>NLGAAVAILGGPGTVQGVVRFLQLTPERCLIEGTIDGLEPGLHGLHVHQYGDLTNNCNSCGNHFNPDGASHGGPQDSDRHRGDLGNVRADADGRAIFRMEDEQLKVWDVIGRSLIIDEGEDDLGRGGHPLSKITGNSGERLACGIIARSAGL[2x]

Superoxide dismutase-1 (SOD1) is one of the most abundant human proteins and is an important part of our antioxidant, redox signalling and respiratory control mechanisms. SOD1 folding, zinc and copper acquisition, and disulphide bond formation can be catalysed by the copper chaperone for SOD1 (CCS), which forms a transient heterodimeric complex with SOD1 to facilitate its maturation. Here, we discover the mechanisms that govern SOD1 maturation and stabilisation through interaction with the chaperone protein hCCS. Combinations of mutants yielded crystallographic structures of full-length hCCS in two different conformers complexed with hSOD1; an hCCS domain II truncation complexed with hSOD1; an hCCS domain II homodimer structure at higher resolution than previously available (1.55 Å); and the hSOD1 disulphide knock-out mutant used to promote complexation.

When homodimeric hSOD1 and hCCS domain II are physiologically zinc metalated, many of the terms that comprise binding free energy are equal due to their sequence and structural similarity. Indeed, orientation of monomers and the presence of four inter-subunit hydrogen bonds found in homodimeric hSOD1 are maintained by hCCS. The presence of a stabilising Coulombic interaction between opposing hCCS Arg104 and Asp136 residues (3.55 Å), which is not present in hSOD1, appears counterintuitive in this regard. However, the hCCS dimer interface is replete with positive charge and therefore not dominated by the hydrophobic effect seen in hSOD1 and many other protein complexes. Most importantly, however, the presence of hCCS Ala231 significantly weakens half of the homodimer interface hydrogen bonds conserved from SOD1. Specifically, Ala231 side-chain methyl pushes Arg232 and Gly135 apart through steric repulsion, lengthening the carbonyl-amine hydrogen bond between them to 3.08 Å from 2.75 Å, in the case of the homologous SOD1 residues Ile151 and Gly51. Without this rearrangement, hCCS Ala231 Cβ would be an energetically unfavourable 2.3 Å from the Gly135 carbonyl oxygen. Introduction of the hCCS Ala231Gly amino acid substitution to mimic the hSOD1 dimer interface increases hCCS dimer affinity, slows complexation with hSOD1 more than 300-fold, impedes hSOD1 activation, and hSOD1 disulphide formation. Thus, relatively weak CCS homodimer affinity has been evolutionarily maintained to provide a pool of monomeric CCS available to interact with and activate nascent monomeric SOD1 within a physiologically relevant timescale. The SOD1-like, hCCS domain II found within each complex structure has an intact intra-subunit disulphide bond in contrast to the yeast orthologue. This disulphide does not dictate complexation but does thermally stabilise the hCCS homodimer and the complex with hSOD1.>[2x]MGMFLFTHKTSAQNIENLSIHQSPTEALDSTFFHHVPLKDYGNLITPSNNTTFTTNYEPSGSSWGEVLDEQNVYLARLKHISNSNNTWDLRIGKGGQIYSFIGPYGEGVPPSSKSHSQWNDEVW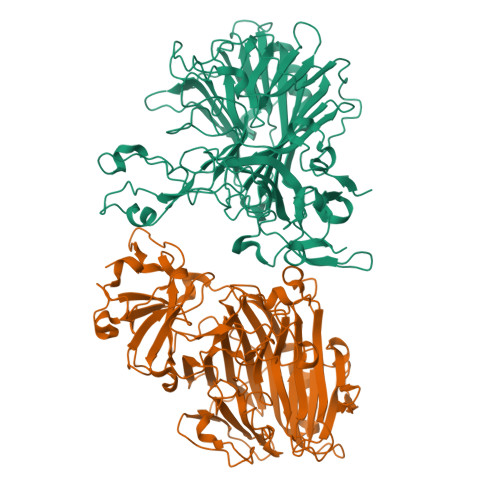QPVSVSGSLNNGDQNDELKEGATNAGLKYFIHGAGTYLTEGLDTPFYSPLMASYYNPTEKAYYVTNWGAQAHLPSLFKSGVLYTTKYKDIGEGILEVTYVIENFGTDTLDHLNIPWGGVRSSSLRGKFVSRPGGDIEIIYGQTGTDNAGDLEDIDATGGYVIYAQDTLSASSPALGIVFGDKILTEEFSDHDLTRIYYRSAQVGGDTNPRDYTLFTTIAKIDVKPKDIFYYRIYYINGTREEVQEKANKIKSEVAYGFITPTIENTSMVTIKNEELDDALNQDIQLFTSPVKGMVPIFLMRNTTTGKEYISPDLYYDIDTFPFSNPYEEDSPKYETYQNRITYRQYNGKIEYIRLLGYASNEDLSNEETQYTLLDNLIVDNTKVVLTTEYLNKLWVPLYHHHHHH>MRKILITGGAGFIGSALVRYIINETSDAVVVVDKLTYAGNLMSLAPVAQSERFAFEKVDICDRAELARVFTEHQPDCVMHLAAESHVDRSIDGPAAFIETNIVGTYTLLEAARAYWNALTEDKKSAFRFHHISTDEVYGDLHSTDDFFTETTPYAPSSPYSASKASSDHLVRAWLRTYGLPTLITNCSNNYGPYHFPEKLIPLMILNALAGKSLPVYGNGQQIRDWLYVEDHARALYCVATTGKVGETYNIGGHNERKNLDVVETICELLEELAPNKPHGVAHYRDLITFVADRPGHDLRYAIDASKIARELGCVPQET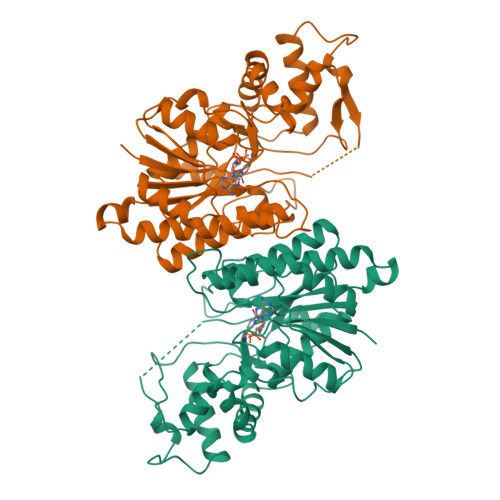FESGMRKTVQWYLANESWWKQVQDGSYQGERLGLKG[2x]(3R)-1-(7H-pyrrolo[2,3-d]pyrimidin-4-yl)piperidin-3-amine 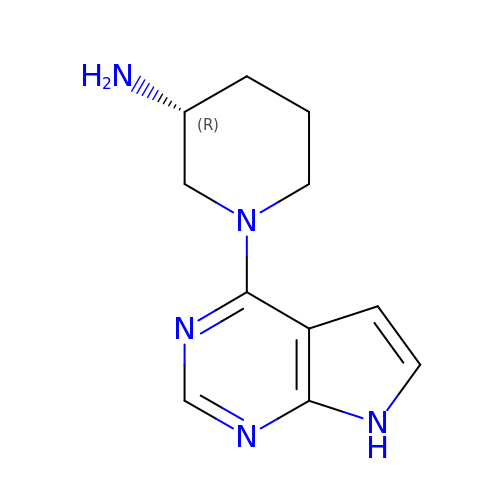| C11 H15 N5 | RAXIOGMWIDLDQC-MRVPVSSYSA-N>[178x]SKTIVLSVGEATRTLTEIQSTADRQIFEEKVGPLVGRLRLTASLRQNGAKTAYRVNLKLDQADVVDCSTSVCGELPKVRYTQVWSHDVTIVANSTEASRKSLYDLTKSLVATSQVEDLVVNLVPLGR;>LEEHYYSRKTCGSGGGLSVQRTGYPQTDPPVFKAVNSFERAPLIVGDHVHSLPYWSRKITLECTPYPFTLRWEGGVHKDGIPDKVPHPSCDPG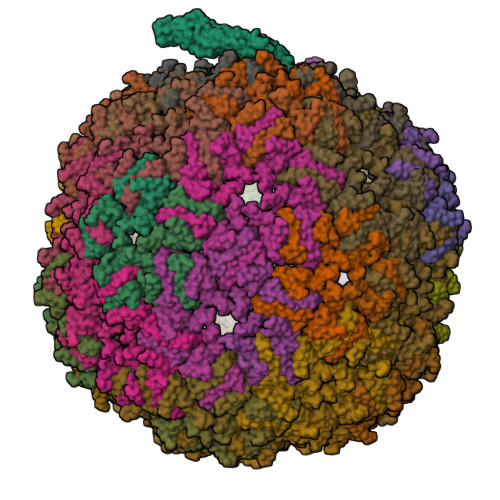SELVSYTHSREVDCERFIGPVPSSFTDPKVTSAQWKFLEDMADMKALADLNKSLVNLPMLYKERRETLKMVGNRLGGLVRVAHAAQDRDLKRYFKARRKDRRKVAEEVANGHLELIFGWLPLIGELEGAIEYAELPDLDFIRCHGLHTLVLQSTPWDNSVDVRSYPNWERAAGTRITGSVRTRGVVESRASVRTALRFNLETSLAGDARRLGFEPISTTYDMIPLSFVVGWFSNFDKYVRTLAPLIGVTFETGSQNRRTTCELVGCTRFYPRTVSPPSGWFARWKDFPDGSLSEVSGLRRTDIRSVLSTLPDPDVRFHADVGLFEISAGISLLAQRYLKPLQRLLKRKSFFYGRT[2x]>GSHMGGERTVTIRRQTVGGFGLSIKGGAEHNIPVVVSKISKEQRAELSGLLFIGDAILQINGINVRKCRHEEVVQVLRNAGEEVTLTVSFLKRAPGSAYGSVKAYTNFDAERDALNIETAIKTKGVDEVTIVNILTNRSNEQRQDIAFAYQRRTKKELASALKSALSGHLETVILGLLKTPAQYDASELKASMKGLGTDEDSLIEIICSRTNQELQEINRVYKEMYKTDLEKDIISDTSGDFRKLMVALAKGRRAEDGSVIDYELIDQDARDLYDAGVKRKGTDVPKWISIMTERSVPHLQKVFDRYKSYSPYDMLESIRKE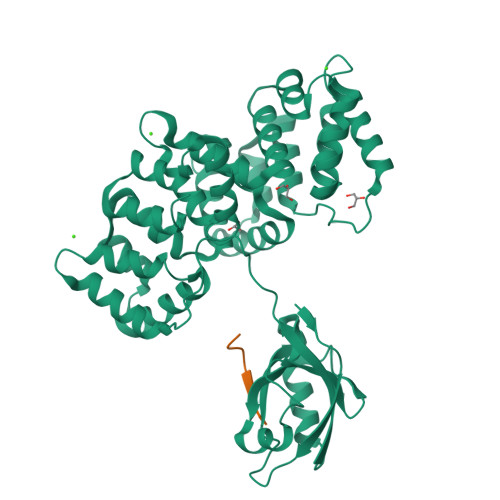VKGDLENAFLNLVQCIQNKPLYFADRLYDSMKGKGTRDKVLIRIMVSRSEVDMLKIRSEFKRKYGKSLYYYIQQDTKGDYQKALLYLCGGDD[2x];>RVRKLPETTL[2x]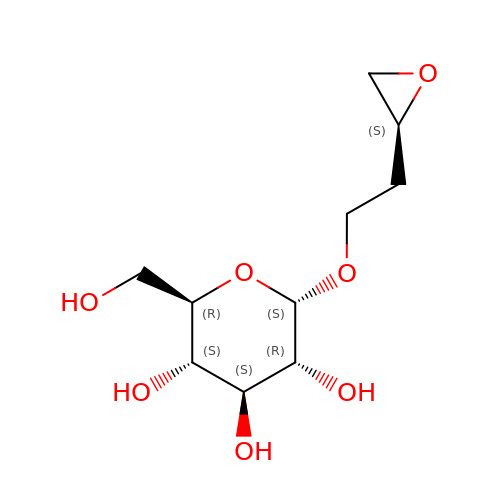2-[(2S)-oxiran-2-yl]ethyl alpha-D-glucopyranoside | C10 H18 O7 | RZSIARIQGABJJE-DLXYEPTOSA-N>GSHMVMNTHPYQSEAVSDVWSLSKTSMTFQPKKASLQPLTISLDELFSSRGEFISVGGNGRMSHKEAILLGLRYKKLYNQARVKYSL[5x];>[5x]SVTVKRIIDNTVIVPKLPANEDPVEYPADYFRKSKEIPLYINTTKSLSDLRGYVYQGLKSGNVSIIHVNSYLYGALKDIRGKLDKDWSSFGINIGKAGDTIGIFDLVSLKALDGVLPDGVSDASRTSADDKWLPLYLLGLYRVGRTQMPEYRKKLMDGLTNQCKMINEQFEPLVPEGRDIFDVWGNDSNYTKIVAAVDMFFHMFKKHECASFRYGTIVSRFKDCAALATFGHLCKITGMSTEDVTTWILNREVADEMVQMMLPGQEIDKADSYMPYLIDFGLSSKSPYWSVKNPAFHFWGQLTALLLRSTRARNARQPDDIEYTSLTTAGLLYAYAVGSSADLAQQFCVGDNKYTPDDSTGGLTTNAPPQGRDVVEWLGWFEDQNRKPTPDMMQYAKRAVMSLQGLREKTIG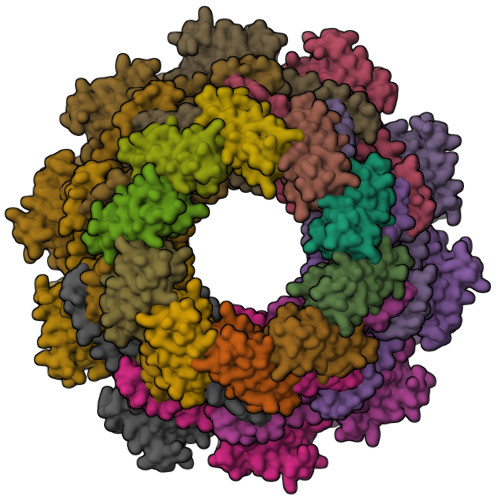KYAKSEFDK>[2x]GAMADIGSMDVLEYFERLKNRELAFVLDDLQLSDMVTRRGFSVIPFDDF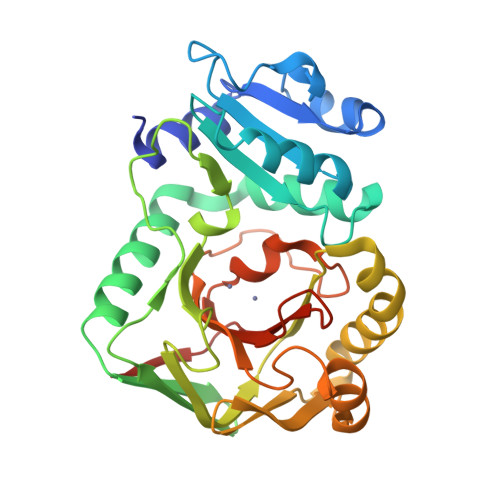DLAREDHPPAFVLVTRLDYHGKLMQAWETAKGISSHLSLAKFDTSPKSVEYSLDQLLSMDFAETLKRRGDYYDSVASTNRMEVVTPGAVLTCDFGNEIEIANNDVEMQKGWLYSVAEFFETSVINLEADRSSYTLNGDLCFTGLIYLCNRPDLKERASATMDELMRMSTRGRNVVSFVDNQIVRMELGGVDMTATLRELIVGKEREGSSTEFAMGCVEYPLAQDWTINSVMNEGSHGIHVGVGMGKEIPHMDFIAKGAELRIAESSDA>[2x]MKKVALVTGAGQGIGKAIALRLVKDGFAVAIADYNDATAKAVASEINQAGGHAVAVKVDVSDRDQVFAAVEQARKTLGGFDVIVNNAGIAQIKPLLEVTEEDLKQIYSVNVFSVFFGIQAAVEAFKKEGHGGKIINAASIAAIQGFPILSAYSTTKFAVRGLTQTAARDLAPLGITV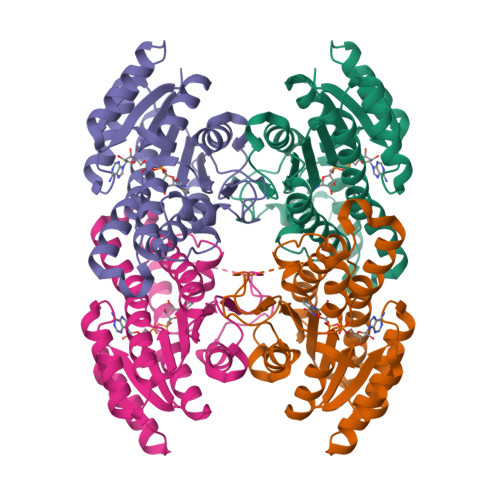NGYCPGIVGTGMWEQIDAELSKINGKPIGENFKEYSSSIALGRPSVPEDVAGLVSFLASPDSDYMTGQSLLIDGGMVFN> PTNYEYDEASETWPSFILTGLLMVVGPMTLLQIYQIFFGANAEDGNSGKSKEFNEEVFKNLNEEYTSDEIKQFRRKFDKNSNKKSKIWSRRNIIIIVGWILVAILLQRINSNDAIKDAATKLFDPYEILGISTSASDRDIKSAYRKLSV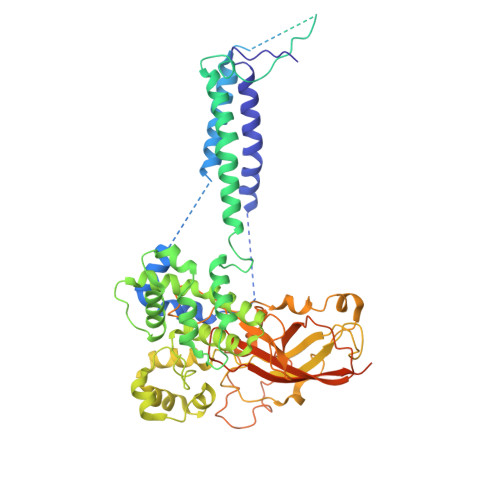KFHPDKLAKGLTPDEKSVMEETYVQITKAYESLTDELVRQNYLKYGHPDGPQSTSHGIALPRFLVDGSASPLLVVCYVALLGLILPYFVSRWWARTQSYTKKGIHNVTASNFVSNLVNYKPSEIVTTDLILHWLSFAHEFKQFFPDLQPTDFEKLLQDHINRRDSGKLNNAKFRIVAKCHSLLHGLLDIACGFRNLDIALGAINTFKCIVQAVPLTPNCQILQLPNVDKEHFITKTGDIHTLGKLFTLEDAKIGEVLGIKDQAKLNETLRVASHIPNLKIIKADFLVPGENQVTPSSTPYISLKVLVRSAKQPLIPTSLIPEENLTEPQDFESQRDPFAMMSKQPLVPYSFAPFFPTKRRGSWCCLVSSQKDGKILQTPIIIEKLSYKNLNDDKDFFDKRIKMDLTKHEKFDINDWEIGTIKIPLGQPAPETVGDFFFRVIVKSTDYFTTDLDITMNMKVRDSPAVEQVEVYSEEDDEYSTDDDETESDDESDASDYTDIDTDTEAEDDESPE>GSMTDGDYDYLIKLLALGDSGVGKTTFLYRYTDNKFNPKFITTVGIDFREKRVVYDTQGADGASGKAFKVHLQLWDTAGLERFRSLTTAFFRDAMGFLLMFDLTSQQSFLNVRNWMSQLQANAYCENPDIVLIGNKADLPDQREVNERQARELAEKYGIPYFETSAATGQNVEKSVETLLDLIMKRMEKCVEKTQVPDTVNGG[2x];>GSSGSSGMGKRLDLSTLTDEEAEHVWAVVQRDFDLRRREEERLQGLKGKIQKESSKRELLSDTAHLNETHCARCLQPYRLLLNSRRQCLECSLFVCKSCSHAHPEEQGWLCDPCHLARVVKIGSLEWYYQHVRA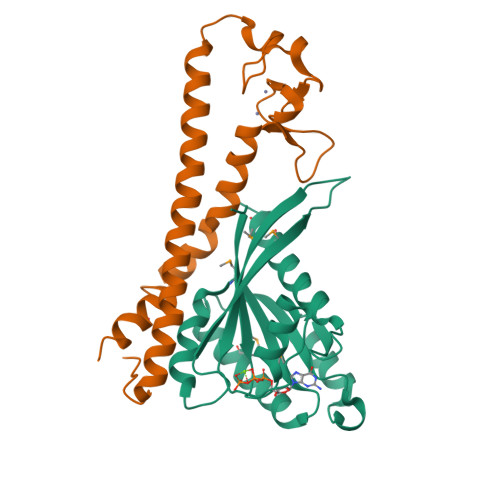RFKRFGSAKVIRSLCGRLQ[2x]> ESQPDPMPDDLHKSSEFTGTMGNMKYLYDDHYVSATKVKSVDKFLAHDLIYNISDKKLKNYDKVKTELLNEDLAKKYKDEVVDVYGSNYYVNCYFSSKDGKVTGGKTCMY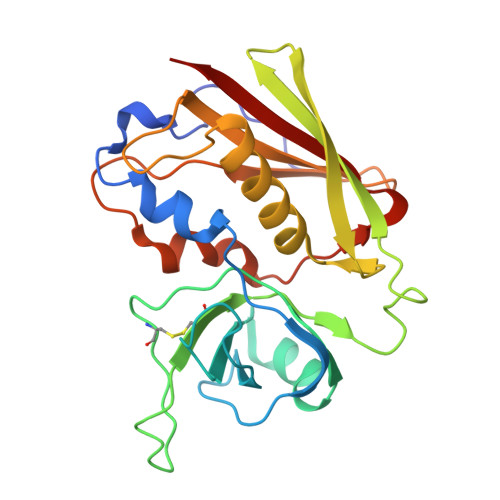GGITKHEGNHFDNGNLQNVLVRVYENKRNTISFEVQTDKKSVTAQELDIKARNFLINKKNLYEFNSSPYETGYIKFIENNGNTFWYDMMPAPGDKFDQSKYLMMYNDNKTVDSKSVKIEVHLTTKNG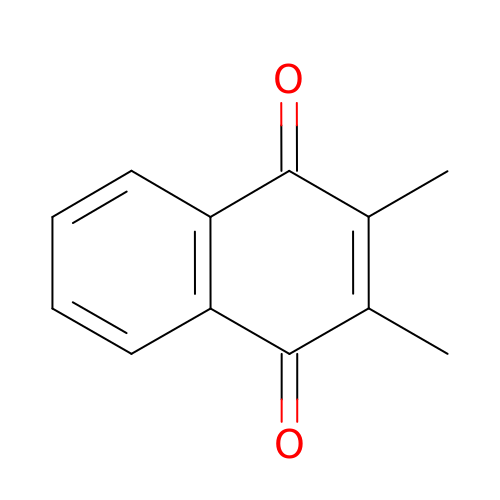2,3-DIMETHYL-1,4-NAPHTHOQUINONE | C12 H10 O2 | LGFDNUSAWCHVJN-UHFFFAOYSA-N>GPGSEEVKKAEESESKSAAKMWENMYKELDRDYSLLEKTVENMSLENMENLDKLNKENQGKLEKLELDYLKKLDHEHKEHQKEQQEQEERQKNQEQLERQSQRE[2x];> GPGSNCGPPPTLSFAAPMDITLTETRFKTGTTLKYTCLPGYVRSHSTQTLTCNSDGEWVYNTFCIYKRCRHPGELRNGQVEIKTDLSFGSQIEFSCSEGFFLIGSTTSRCEVQDRGVGWSHPLPQCEI

Antigenically sequence variable M proteins of the major bacterial pathogen Streptococcus pyogenes (Strep A) are responsible for recruiting human C4b-binding protein (C4BP) to the bacterial surface, which enables Strep A to evade destruction by the immune system. M proteins form parallel, dimeric α-helical coiled coils which are attached to the bacterial cell wall and extend ∼500 Å into the extracellular space. The most sequence divergent portion of M proteins, the hypervariable region (HVR), is responsible for binding C4BP. We identified C4BP-binding in several M proteins that lack an M2 or M22 pattern, and determined the structures of two, M68 and M87 protein HVRs, in complex with C4BPα1-2.

The structure of the complex between M68N100 and C4BPα1-2 was determined to 2.5 Å resolution limit by multiwavelength anomalous dispersion phasing using selenomethionine (SeMet)-labeled M68N100. The architecture of the complex differed substantially from that of M87 protein and those observed previously. M68N100 formed an α-helical dimer but not a coiled coil. The two M68 helices were asymmetrically disposed and mostly parallel to one other, except for the very N-terminal segment (aa 42–77), where one of the helices wrapped around the other. About two heptads of this N-terminal segment (aa 58–70) bound C4BP. Only a single C4BPα1-2 molecule was evident, and in this molecule the C4BPα1 domain was largely disordered. The C4BPα2 quadrilateral contacted M68 protein, although with some variations. The C4BPα2 quadrilateral hydrophobic pocket (ΦHis 67), instead of contacting a single hydrophobic M protein amino acid, contacted a cluster: M68 Met 58, Trp 59, and Met 62 from one helix and Tyr 63, along with the alkyl chain of K64, from the second. Valine substitution of M68 W59 or Y63 reduced C4BP binding ∼50-fold relative to WT M68 protein. In contrast, the M68 HVR utilized the C4BPα2 quadrilateral, albeit using multiple amino acids rather than a single one to contact the ΦHis 67 site, but lacked contact to the C4BPα1 Arg39 nook, with the C4BPα1 domain in this complex almost entirely disordered.[(2R,3S,4R,5R)-5-(6-amino-9H-purin-9-yl)-3,4-dihydroxytetrahydrofuran-2-yl]methyl (2R,3S,4S)-5-[(3R,3aS,7aR)-10,11-dimethyl-1,4,6-trioxo-3-phenyl-2,3,5,6,7,7a-hexahydro-1H-benzo[g]pyrrolo[2,1-e]pteridin-8(4H)-yl]-2,3,4-trihydroxypentyl 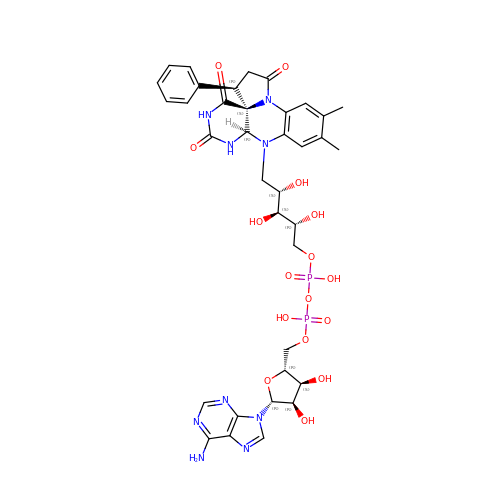dihydrogen diphosphate | C36 H43 N9 O16 P2 | QWOOVYWBGZGGNV-ITRBMUPBSA-N>[4x]ATMKYVGS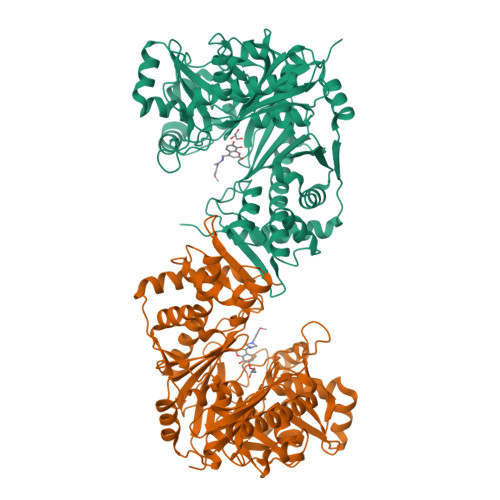IDQGTTSTRFIIFDERQRPVSVHQVPHTQHTPHPGWLEHDPMEIFRSACKCMSVAIAKLRQKDASFRKIEAIGITNQRETTVAWDRVTKEPLCYAPVWNDLRTYDITKKVTAELGGGDSMFASKITGLPVSTYFAAFKMRWMLENVPAVADACRRGTLCFGTIDTWLMYKLSGGKAFVTDVTNASRTFLMDLRTRKWSPELCEKLKIPMETLPEIRSNSELFGYVETDECGVAAALNERTPIMGSIGDQQSALFGNMCFEKGEAKNTYGTGCFLLMNVGEEARFSKHGLLSTVGFQVGRDGPCYYALEGAIACAGATVEWMRRNMNLFSHITECEKLARSVPGTQGIVFVPAFSGLLAPYWDPSARGTIVGMTLKTTRAHVIRAALQAIALQLNDVVGSMKRDAGLNLSSLRVDGGLSKNGLLMEIQASLLGVDILVPSMHETTALGAALCAGLAAGVWTSLEEVKAVSRRENSWKTVSPSGSAMEREAMIAEWREALKRTKWAKL>MGFTIDIKSFLKPGEKTYTQR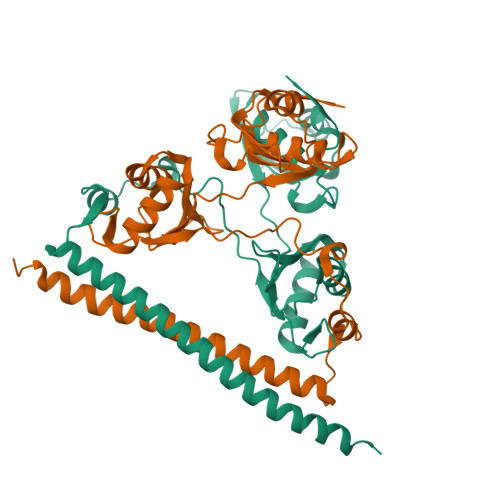CRLFVGNLPTDITEEDFKRLFERYGEPSEVFINRDRGFGFIRLESRTLAEIAKAELDGTILKSRPLRIRFATHGAALTVKNLSPVVSNELLEQAFSQFGPVEKAVVVVDDRGRATGKGFVEFAAKPPARKALERCGDGAFLLTTTPRPVIVEPMEQFDDEDGLPEKLMQKTQQYHKEREQPPRFAQPGTFEFEYASRWKALDEMEKQQREQVDRNIREAKEKLEAEMEAARHEHQLMLM[2x]> MVAVERVESLAKSGIISIPKEYIRPKEELESINDVFLEEKKEDGPQVPTIDLKNIESDDEKIRENCIEELKKASLDWGVMHLINHGIPADLMERVKKAGEEFFSLSVEEKEKYANDQATGKIQGYGSKLANNASGQLEWEDYFFHLAYPEEKRDLSIWPKTPSDYIEATSEYAKCLRLLATKVFKALSVGLGLEPDRLEKEVGGLEELLLQMKINYYPKCPQPELALGVEAHTDVSALTFILHNMVPGLQLFYEGKWVTAKCVPDS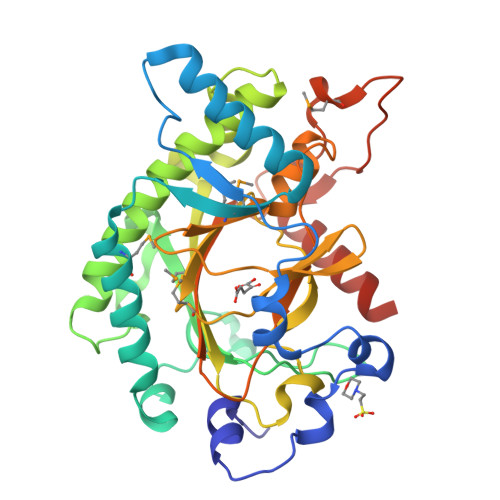IVMHIGDTLEILSNGKYKSILHRGLVNKEKVRISWAVFCEPPKDKIVLKPLPEMVSVESPAKFPPRTFAQHIEHKLFGKEQEELVSEKND> MANASGNMSAVRETMDVLLEISRLLNT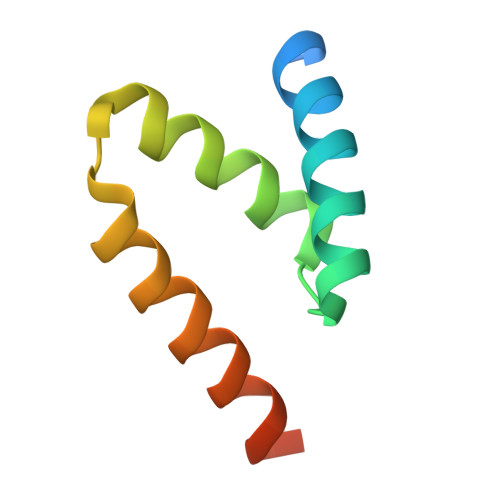GLDMETLSICVRLCEQGINPEALSSVIKELRRASDTLKASESTAS>MGRMLGRKERTL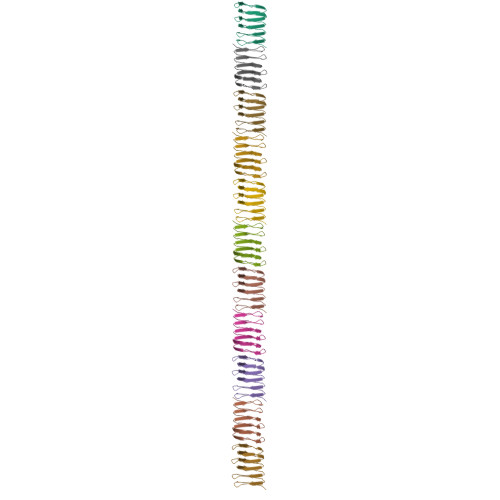TYLGPDTEVLGDMRAKGQVRIDGLVRGSVLVEGELEVGPTGRVEGERVEARSVLIHGEVKAELTAEKVVLSKTARFTGQLKAQALEVEAGAVFVGQSVAGEHKALEAPKEA[22x]> LPTQPRDIENFNSTQKFIEDNIEYITIIAFAQYVQEATFEEMEKLVKDMVEYKDRCMADKTLPECSKLPNNVLQEKICAMEGLPQKHNFSHCCSKVDAQRRLCFFYNKKSDVGFLPPFPTLDPEEKCQAYESNRESLLNHFLYEVARRNPFVFAPTLLTVAVHFEEVAKSCCEEQNKVNCLQTRAIPVTQYLKAFSSYQKHVCGALLKFGTKVVHFIYIAILSQ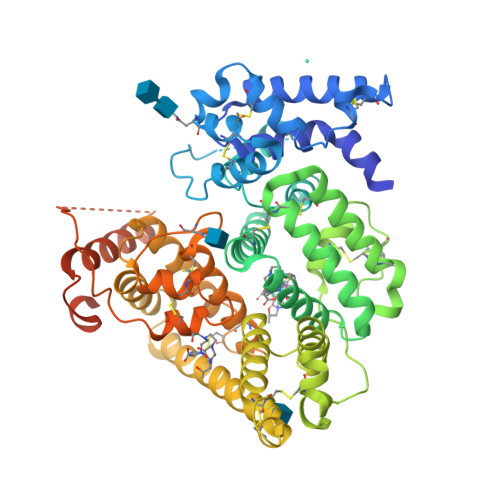KFPKIEFKELISLVEDVSSNYDGCCEGDVVQCIRDTSKVMNHICSKQDSISSKIKECCEKKIPERGQCIINSNKDDRPKDLSLREGKFTDSENVCQERDADPDTFFAKFTFEYSRRHPDLSIPELLRIVQIYKDLLRNCCNTENPPGCYRYAEDKFNETTEKSLKMVQQECKHFQNLGKDGLKYHYLIRLTKIAPQLSTEELVSLGEKMVTAFTTCCTLSEEFACVDNLADLVFGELCGVNENRTINPAVDHCCKTNFAFRRPCFESLKADKTYVPPPFSQDLFTFHADMCQSQNEELQRKTDRFLVNLVKLKHELTDEELQSLFTNFANVVDKCCKAESPEVCFNEESPKIGNKGENLYFQ> MGSAMSLGCSKRKATNQDVDSESRKRRKICSTNDAENCRFIQDESSWKHPWSLCANSVVNDTKDTKSSALSLPSPPTSVSRIWKHQVFPSFHGADVRKTILSHILESFRRKGIDPFIDNNIERSKSIGHELKEAIKGSKIAIVLLSKNYASSSWCLDELAEIMKCRELLGQIVMTIFYEVDPTDIKKQTGEFGKAFTKTCKGKTKEYVERWR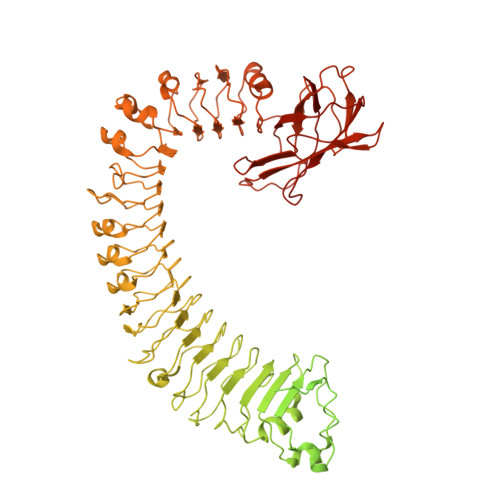KALEDVATIAGYHSHKWRNEADMIEKIATDVSNMLNSFKPSRDFNGLVGMRAHMDMLEQLLRLVLDEVRMIGIWGPPGIGKTTIARFLFNQVSDRFQLSAIMVNIKGCYPRPCFDEYSAQLQLQNQMLSQMINHKDIMISHLGVAQERLRDKKVFLVLDEVDQLGQLDALAKETRWFGPGSRIIITTEDLGVLKAHGINHVYKVGYPSNDEAFQIFCMNAFGQKQPHEGFDEIAREVMALAGELPLGLKVLGSALRGKSKPEWERTLPRLKTSLDGKIGSIIQFSYDALCDEDKYLFLYIACLFNKESTTKVEGLLGKFLDVRQGLHILAQKSLISIEDGNIYMHTLLEQFGRETSRKQFIHHGYTKHQLLVGERDICEVLNDDTIDSRRFIGINLDLYKNVEELNISEKALERIHDFQFVRINGKNHALHERLQGLIYQSPQIRSLHWKCYQNICLPSTFNSEFLVELDMSFSKLQKLWEGTKQLRNLKWMDLSYSSYLKELPNLSTATNLEELKLRNCSSLVELPSSIEKLTSLQILDLHRCSSLVELPSFGNATKLEILNLENCSSLVKLPPSINANNLQELSLTNCSRVVELPAIENATNLWKLNLLNCSSLIELPLSIGTATNLKHLDFRGCSSLVKLPSSIGDMTNLEVFYLSNCSNLVELPSSIGNLRKLTLLLMRGCSKLETLPTNINLKSLHTLNLIDCSRLKSFPEISTHIKYLRLIGTAIKEVPLSIMSWSPLAHFQISYFESLKEFPHALDIITELQLSKDIQEVPPWVKRMSRLRALRLNNCNNLVSLPQLPDSLAYLYADNCKSLERLDCCFNNPEIRLYFPKCFKLNQEARDLIMHTSTRNFAMLPGTQVPACFNHRATSGDSLKIKLKESPLPTTLTFKACIMLVNEEMSYDLKSMSVDIVIRDEQNDLKVQCTPSYHQCTEIYVLTEHIYTFELEVEEVTSTELVFEFTSVNESICKIGECGILQRETRSLRRSSSPDLSPESSRVSSCDHC>MAHHHHHHMILK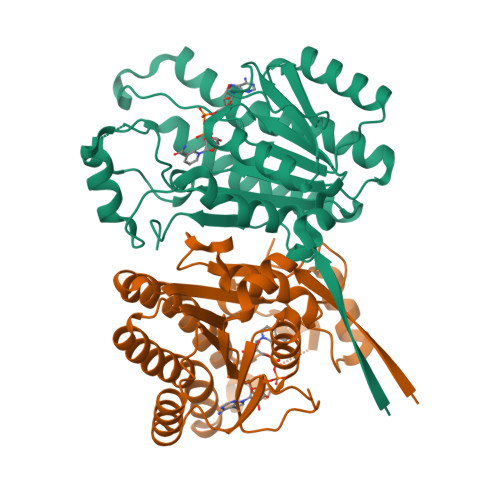NFSDEFQDKLVLITGGSGQIGSELVESYLSVSARVICLDPEQPSVDYKSNRFEWIQADITNRKEIKEIFLSLENQNKIPDILINCAGISVFTPFEDRTDEEFNEVVHVNLNGTFLLSQYTFRLWKEKGKKGIILNFGSIYGVSIADMRIYGDSGRNSPEVYAMTKAGIIHFTKYLARYAAPYGIRVNCISPGGIFANQSSDFIQNYIYKTPLGRMGNPSDLVGGVFFLTSSLSEYVTGQNLLIDGGFTIGD[2x]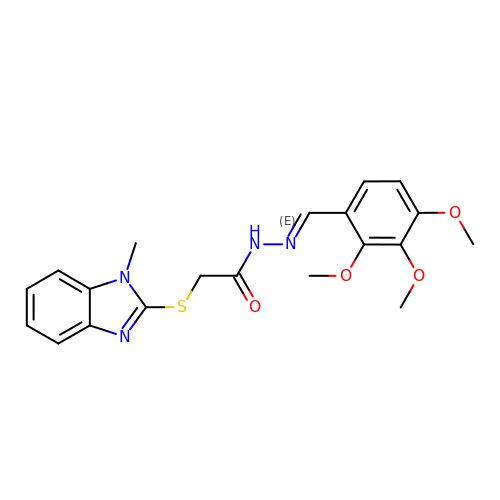2-(1-methylbenzimidazol-2-yl)sulfanyl-N-[(E)-(2,3,4-trimethoxyphenyl)methylideneamino]ethanamide | C20 H22 N4 O4 S | CKRLLWUTMXLHQI-SRZZPIQSSA-N> MPTNYEYDEASETWPSFILTGLLMVVGPMTLLQIYQIFFGANAEDGNSGKSKEFNEEVFKNLNEEYTSDEIKQFRRKFDKNSNKKSKIWSRRNIIIIVGWILVAILLQRINSNDAIKDAATKLFDPYEILGISTSASDRDIKSAYRKLSVKFHPDKLAKGLTPDEKSVMEETYVQITKAYESLTDELVRQNYLKYGHPDGPQSTSHGIALPRFLVDGSASPLLVVCYVALLGLILPYFVSRWWARTQSYTKKGIHNVTASNFVSNLVNYKPSEIVTTDLILHWLSFAHEFKQFFPDLQPTDFEKLLQDHINRRDSGKLNNAKFRIVAKCHSLLHGLLDIACGFRNLDIALGAINTFKCIVQAVPLTPNCQILQLPNVDKEHFITKTGDIHTLGKLFTLEDAKIGEVLG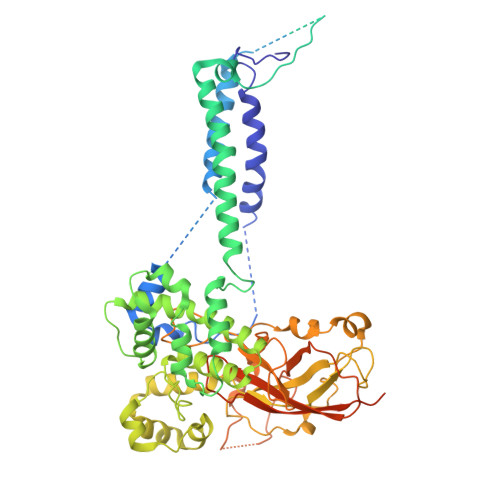IKDQAKLNETLRVASHIPNLKIIKADFLVPGENQVTPSSTPYISLKVLVRSAKQPLIPTSLIPEENLTEPQDFESQRDPFAMMSKQPLVPYSFAPFFPTKRRGSWCCLVSSQKDGKILQTPIIIEKLSYKNLNDDKDFFDKRIKMDLTKHEKFDINDWEIGTIKIPLGQPAPETVGDFFFRVIVKSTDYFTTDLDITMNMKVRDSPAVEQVEVYSEEDDEYSTDDDETESDDESDASDYTDIDTDTEAEDDESPE(E)-4-((1-methylpiperidin-4-yloxyimino)methyl)benzimidamide | C14 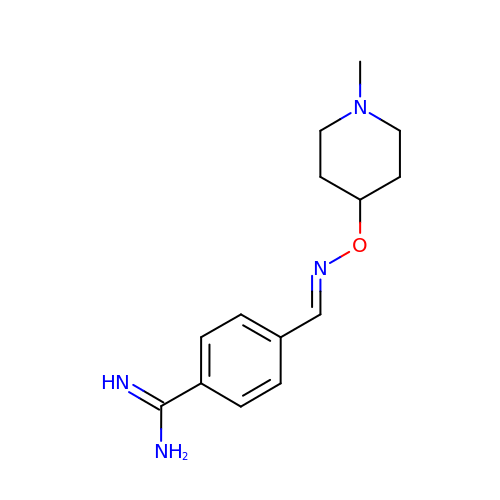H20 N4 O | FNLKRNACHKABQI-LICLKQGHSA-N> MLESKLINHIATQFLDGEKDGLDSQTPLFELNIVDSAAIFDLVDFLRQESKVSIGMQEIHPANFATVQSMVALVQRLKAHPEQGGA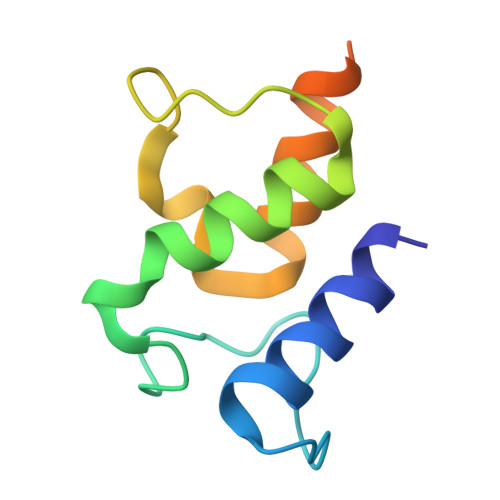AWEHHHHHH We report the 2.3-Å resolution crystal structure of QDE-1, a cRdRP from Neurospora crassa, and find that it forms a relatively compact dimeric molecule, each subunit of which comprises several domains with, at its core, a catalytic apparatus and protein fold strikingly similar to the catalytic core of the DNA-dependent RNA polymerases responsible for transcription. A cell-encoded RNA-dependent RNA polymerase (cRdRP) is also involved, in plants, fungi, protozoa, and certain animals, but apparently not insects and vertebrates, producing dsRNA triggers and hence amplifying the PTGS response. The polypeptide chain then leads into a “catalytic” domain (residues 647–807; 914–1,161) that houses the three proposed catalytic aspartic acid residues (D1007, D1009, and D1011) within an active site cleft formed between two DPBB subdomains (DPBB1, residues 690–792, and DPBB2, residues 916–1,018). Overall, QDE-1 exists as a compact, but flexible, dimeric enzyme with metal binding sites confirming positions of the catalytic sites but with extensive additional structure whose biological functions are less immediately clear.

In addition, a lower resolution structure (3.5-Å resolution) was determined in space group C2. In space group C2, the dimer is formed by two subunits related by exact crystallographic 2-fold symmetry. In the lower resolution C2 crystal form, the molecule forms a symmetric dimer. Here, the subunits both assume a partially closed conformation (the head is rotated by 4° relative to A and 8° to B, and the slab is displaced upwards and outwards by 4° relative to A and 2° to B).

> ESARSQVQVHAPVVAARLRNIWPKFPKWLHEAPLAVAWEVTRLFMHCKVDLEDESLGLKYDPSWSTARDVTDIWKTLYRLDAFRGKPFPEKPPNDVFVTAMTGNFESKGSAVVLSAVLDYNPDNSPTAPLYLVKLKPLMFEQGCRLTRRFGPDRFFEILIPSPTSTSPSVPPVVSKQPAAVEEVIQWLTMGQHSLVGRQWRAFFAKDAGYRKPLREFQLRAEDPKPIIKERVHFFAETGITFRPDVFKTRSVVPAEEPVEQRTEFKVSQMLDWLLQLDNNTWQPHLKLFSRIQLGLSKTYAIMTLEPHQIRHHKTDLLSPSGTGEVMNDGVGRMSRSVAKRIRDVLGLGDVPSAVQGRFGSAKGMWVIDVDDTGDEDWIETYPSQRKWECDFVDKHQRTLEVRSVASELKSAGLNLQLLPVLEDRARDKVKMRQAIGDRLINDLQRQFSEQKHALNRPVEFRQWVYESYSSRATRVSHGRVPFLAGLPDSQEETLNFLMNSGFDPKKQKYLQDIAWDLQKRKCDTLKSKLNIRVGRSAYIYMIADFWGVLEENEVHVGFSSKFRDEEESFTLLSDCDVLVARSPAHFPSDIQRVRAVFKPELHSLKDVIIFSTKGDVPLAKKLSGGDYDGDMAWVCWDPEIVDGFVNAEMPLEPDLSRYLKKDKTTFKQLMASHGTGSAAKEQTTYDMIQKSFHFALQPNFLGMCTNYKERLCYINNSVSNKPAIILSSLVGNLVDQSKQGIVFNEASWAQLRRELLGGALSLPDPMYKSDSWLGRGEPTHIIDYLKFSIARPAIDKELEAFHNAMKAAKDTEDGAHFWDPDLASYYTFFKEISDKSRSSALLFTTLKNRIGEVEKEYGRLVKNKEMRDSKDPYPVRVNQVYEKWCAITPEAMDKSGANYDSKVIRLLELSFLADREMNTWALLRASTAFKLYYHKSPKFVWQMAGRQLAYIKAQMTSRPGEGAPALMTAFMYAGLMPDKKFTKQYVARLEGDGSEYPDPEVYEVLGDDDFDGIGFTGNGDY>[2x]GSHGMPLPATHDIHLHGSINGHEFDMVGGGKGDPNAGSLVTTAKSTKGALKFSPYLMIPHLGYGYYQYLPYPDGPSPFQVSMLEGSGYAVYRVFDFEDGGKLSTEF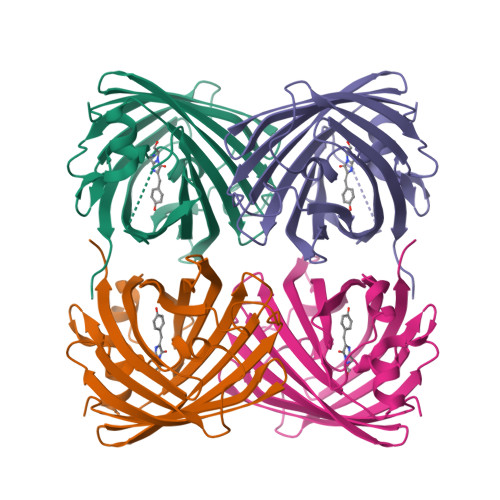KYSYEGSHIKADMKLMGSGFPDDGPVMTSQIVDQDGCVSKKTYLNNNTIVDSFDWSYNLQNGKRYRARVSSHYIFDKPFSADLMKKQPVFVYRKCHVKATKTEVTLDEREKAFYELA> MSTDSAYAVELKGLTFKRGSRAIFDNIDVRIPRGKVTGIMGPSGCGKTTLLRLIASQLRPSKGEVWVNGQNLPQLSRGDLFDMRKQFGV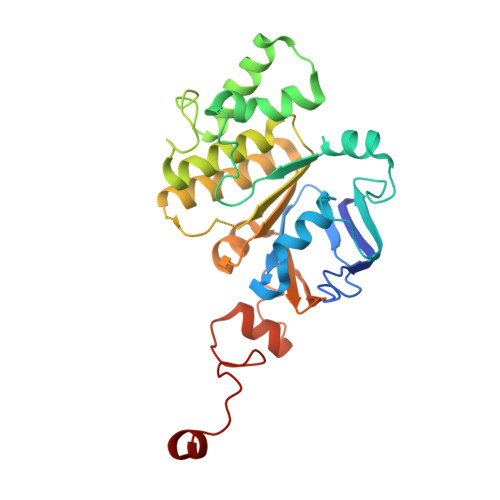LFQSGALFTDLDVFENVAFPLRVHTQLPEEMIRDIVLMKLQAVGLRGAVELMPDELSGGMKRRVALARAIALDPQILLYDEPFVGQDPIAMGVLVRLIRLLNDALGITSIVVSHDLAETASIADYIYIVGDGRVLGHGTPDVLKETDDPRIRQFVKGIPDGPVPFHYPARDYRADLLGER>[2x]ADPLLPYFDFDVPRNLTVTVGQTGFLHCRVERLGDKDVSWIRKRDLHILTAGGTTYTSDQR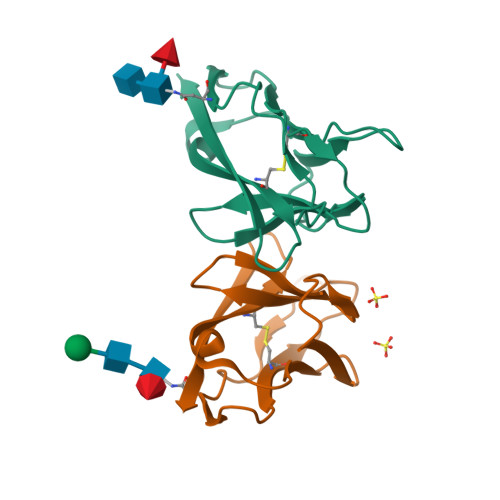FQVLRPDGSANWTLQIKYPQPRDSGVYECQINTEPKMSLSYTFNVVEHHHHHH;>SRIVDPKFSSPIVNMTAPVGRDAFLTCVVQDLGPYKVAWLRVDTQTILTIQNHVITKNQRIGIANSEHKTWTMRIKDIKESDKGWYMCQINTDPMKSQMGYLDVVVHHHHHH[2x]> YEYVELAKASLTSAQPQHFYAVVIDATFPYKTNQERYICSLKIVDPTLYLKQQKGAGD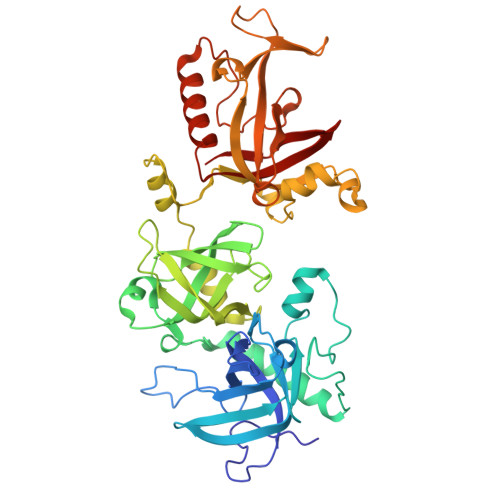ASDYATLVLYAKRFEDLPIIHRAGDIIRVHRATLRLYNGQRQFNANVFYSSSWALFSTDKRSVTQEINNQDAVSDTTPFSFSSKHATIEKNEISILQNLRKWANQYFSSYSVISSDMYTALNKAQAQKGDFDVVAKILQVHELDEYTNELKLKDASGQVFYTLSLKLKFPHVRTGEVVRIRSATYDETSTQKKVLILSHYSNIITFIQSSKLAKELRAKIQDDHSVEVASLKKNVSLNAVVLTEVDKKHAALPSTSLQDLFHHADSDKELQAQDTFRTQFYVTKIEPSDVKEWVKGYDRKTKKSSSLKGASGKGDNIFQVQFLVKDASTQLNNNTYRVLLYTQDGLGANFFNVKADNLHKNADARKKLEDSAELLTKFNSYVDAVVERRNGFYLIKDTKLI>HHHHHHMVTQFKTASEFDSAIAQDKLVVVDFYATWCGPSKMIAPMIEKFSEQYPQADFYKLDVDELGDVAQKNEVSAMPTLLLFKNGKEVAK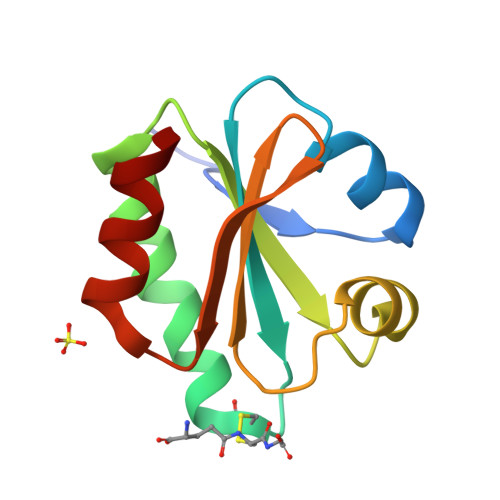VVGANPAAIKQAIAANA[2x]>[2x]MSNVIQFYDIPGNATPDKAWSPNTWKT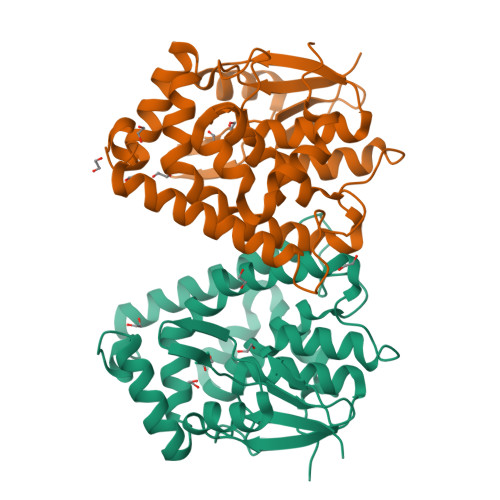RYTLNFKGIPYKTIWVEYPDIASVCKEIGAEPTSIRPDGPYYTLPVIHDPSTGKTISDSAAIARYLDKTYPDTPVVIPPETDALHAAFNFAFSEAIVRALAPIMLPATNAQLNPRSEEFFRRTREESAGGVKLEDWAPPGSEKRAKAWEKIRAGFGQIAKWLSADGNDKLLFLGDKVSYADITIVGWVIWVKRVLGPDSAEWKDFETWDDGKWAKQLALFEKYEVVPDA>[2x]GSPAKIKIVAPLESALIPGGETYQLRCDIMSTPAATIHWKFNGKLIQGSNELNVEEKLLNFGKAIVDTGIVASILTIQCPSAENSGTYSCVGYNGHQTIETVAEVEIEGEASGCRSNHKSAPEIV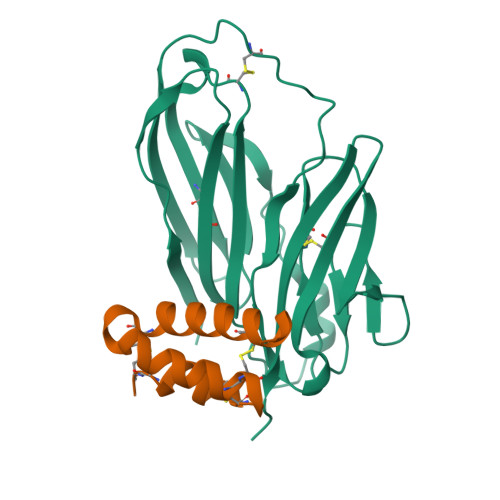FWTDSRFEMTGNVATLVCRANQQVDWVWMSNDELVKNNDKFTVLSNGDLVIKNIVWDDMGTYTCIARNQFGEARQETFLYPTAHHHHHH;>VPAPGETRACGRKLISLVMAVCGDLCNPQEGKDIATECCGNQCSDDYIRSACCPHHHHHH[2x]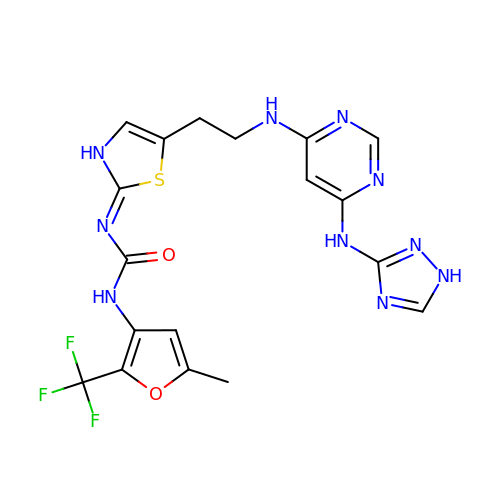1-[5-methyl-2-(trifluoromethyl)furan-3-yl]-3-[(2Z)-5-(2-{[6-(1H-1,2,4-triazol-3-ylamino)pyrimidin-4-yl]amino}ethyl)-1,3-thiazol-2(3H)-ylidene]urea | C18 H17 F3 N10 O2 S | KNTGXMNWVXZIMW-UHFFFAOYSA-N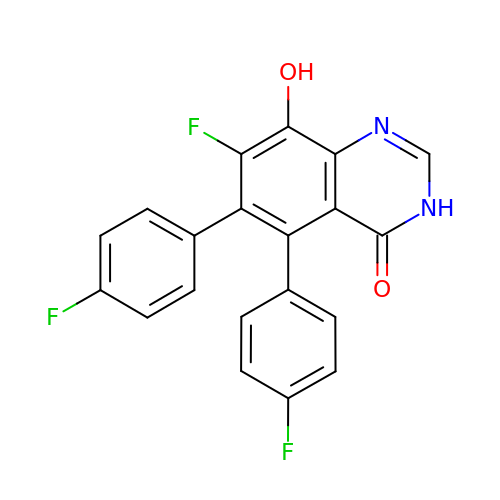7-fluoranyl-5,6-bis(4-fluorophenyl)-8-oxidanyl-3~{H}-quinazolin-4-one | C20 H11 F3 N2 O2 | TXLMFDIODMWHDL-UHFFFAOYSA-N4'-(5-carbamimidoyl-1H-benzimidazol-2-yl)biphenyl-4-carboxamide 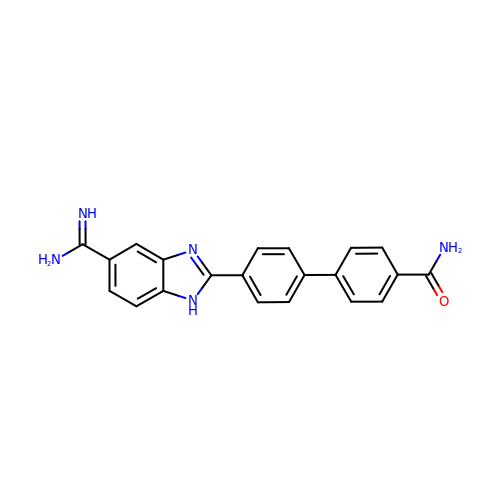| C21 H17 N5 O | LDAVGTBIUFWUTM-UHFFFAOYSA-N>[2x]GSSHHHH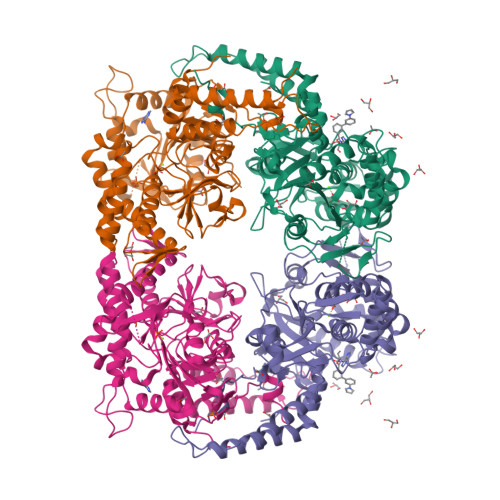HHSSGLVPRGSMSTSWSDRLQNAADMPANMDKHALKKYRREAYHRVFVNRSLAMEKIKCFGFDMDYTLAVYKSPEYESLGFELTVERLVSIGYPQELLSFAYDSTFPTRGLVFDTLYGNLLKVDAYGNLLVCAHGFNFIRGPETREQYPNKFIQRDDTERFYILNTLFNLPETYLLACLVDFFTNCPRYTSCETGFKDGDLFMSYRSMFQDVRDAVDWVHYKGSLKEKTVENLEKYVVKDGKLPLLLSRMKEVGKVFLATNSDYKYTDKIMTYLFDFPHGPKPGSSHRPWQSYFDLILVDARKPLFFGEGTVLRQVDTKTGKLKIGTYTGPLQHGIVYSGGSSDTICDLLGAKGKDILYIGDHIFGDILKSKKRQGWRTFLVIPELAQELHVWTDKSSLFEELQSLDIFLAELYKHLDSSSNERPDISSIQRRIKKVTHDMDMCYGMMGSLFRSGSRQTLFASQVMRYADLYAASFINLLYYPFSYLFRAAHVLMPHESTVEHTHVDINEMESPLATRNRTSVDFKDTDYKRHQLTRSISEIKPPNL> MASMERFLSVYDEVQAFLLDQLQSKYEIDPNRARYLRIMMDTTCLGGKYFRGMTVVNVAEGFLAVTQHDEATKERILHDACVGGWMIEFLQAHYLVEDDIMDGSVMRRGKPCWYRFPGVTTQCAINDGIILKSWTQIMAWHYFADRPFLKDLLCLFQKVDYATAVGQMY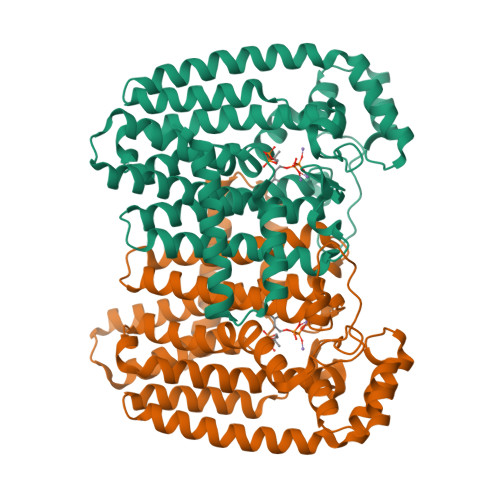DVTSMCDSNKLDPEVAQPMTTDFAEFTPAIYKRIVKYKTTFYTYLLPLVMGLLVSEAAASVEMNLVERVAHLIGEYFQVQDDVMDCFTPPEQLGKVGTDIEDAKCSWLAVTFLGKANAAQVAEFKANYGEKDPAKVAVVKRLYSKANLQADFAAYEAEVVREVESLIEQLKVKSPTFAESVAVVWEKTHKRKK 5'-O-(N-(L-Leucyl)-Sulfamoyl)Cytidine | C15 H25 N5 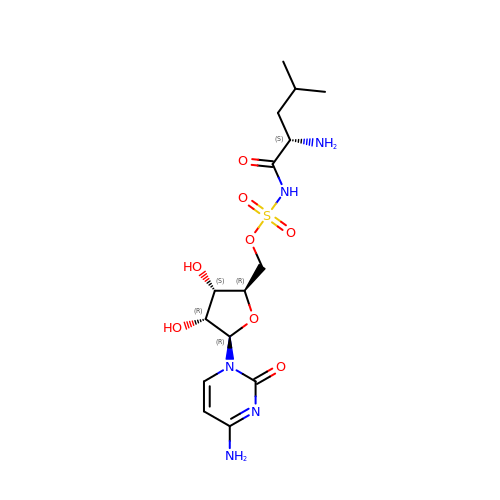O8 S | GAMJBGGTDXDZPE-XKYXEJCGSA-N> SPTPLPQLPSNVRDGENNVASTFLQAFFQLWDHDRLTLIPQFYDSETTFSVVFATDSPQDPASSSCSKFSRNLNILSPRHPSTLQRLFVGSNLIADLWKVLPATRHPSLDQTSQWLIDCHTFPHLADPTGMAPYAMGLMINVNGQCEEADISQNLYGTRTFSRCFILGPSKPGAPHPYRVLSDQLTLHTWKPQ;> MLSRRYAAKSFVEWYYRQINENKPVASGYVNNNATYTKAGHPPADITINGRVVATPEEWDTMLKEQRAQHNTSSSSTLPIGRKPVRYDVDCFDVHVINADYRFAAPQRMIEQHAPTDGVRMMMALTVSGSVYFGASPRSTDDYVIKQHFNDVFILVPNWDVLEKPGARSGRKYLIASHKYRAY;> MMAPANNPFGAPPAQVNNPF

The TREX-2 complex integrates mRNA nuclear export into the gene expression pathway and is based on a Sac3 scaffold to which Thp1, Sem1, Sus1, and Cdc31 bind. TREX-2 also binds the mRNA nuclear export factor, Mex67:Mtr2, through the Sac3 N-terminal region (Sac3N). Whereas protein transport is generally facilitated by karyopherin-β family proteins, mRNA export in yeast is mediated primarily by the Mex67:Mtr2 complex or in metazoans by NXF1:NXT1 (Segref et al., 1997; Braun et al., 2001). Mex67 is a modular protein containing four domains: RNA-recognition motif (RRM), leucine-rich repeat (LRR), nuclear transport factor 2-like (NTF2L), and ubiquitin-associated (UBA).

Diffraction quality crystals were obtained with ctSac31−20 and ctSac320−40. The complex with ctSac31−20 crystallized with P21 symmetry and the structure was determined to 1.8 Å resolution with Sac3 residues 15–20 (QVNNPF) clearly visible in the electron density, whereas the complex with ctSac320−40 crystallized with P212121 symmetry and the structure was determined to 1.85 Å with Sac3 residues 30–37 (SSVFGAPA) built into the model. Both crystal structures also contained the ctMex67 NTF2-like domain together with ctMtr2 and were refined to an Rfree of 19.3% and 20.3%, respectively, with excellent geometry. The Sac3N motifs bind primarily to the Mex67 NTF2L domain, and crystal structures of complexes between Mex67NTF2L:Mtr2 and Sac3N peptides identify a central role of the motif's Phe residue binding into a hydrophobic pocket on Mex67NTF2L. (2001) to which a PGFGQ peptide derived from nucleoporin NUP214 bound to NXF1, albeit with the chain direction reversed. This cavity was formed principally by Gly500, Leu501, Leu530, and Gly531, and accommodated a single Phe residue from either peptide (Phe20 and Phe33) with neighboring residues forming several direct and water-mediated hydrogen bonds. In addition to the hydrophobic interactions dominated by the Phe side chain, putative H bonds were found between the main-chain amino group of Asn380Mex67 and the carbonyl group of the Sac3 Phe. Asn380 also formed putative H bonds with the residue N-terminal to the bound Phe residue (Val32 or Pro19). Although the overall fold of the ctMex67 NTF2L domain or ctMtr2 was not altered by the binding of either ctSac3 peptide, a translation of the loop region of ∼3.0 Å prior to helix α1 of the NTF2L domain (residues 376–382, the pre-α1 loop) was observed for both peptides. However, in the ctSac3 peptides in the present study, a greater contribution was made by residues neighboring the bound Phe; as a result, this residue only contributed to 39% (ctSac31−20) and 35% (ctSac320−40) of the buried surface area.>MTTRTTDNPWLDARVLNMAHAGGENEAPANTLYAFKRAVKLGANMLELDVQSTKDDQLVVIHNATVDQTTDGTGKVRDLTFEQVHELDAAYNFIPGRHAVPGEPPESYPLRGVRTGEKKPPPGYQPSDFAIPKLADVLEAFPRTPINIEIKGTSDADIPSFLHNAKLLARLLKKTGRTDFIVTSLNDLAVAKFHLLAPDIPIAPGMAGLAAYFLLGVKPMHGTVALQIPVRYQGLEIATPEFIRRAHADGYAVHVWFSGTAPDDEATYNRIIDSCADGLMPAYPALLERILDERGIERPGRPGVDPCG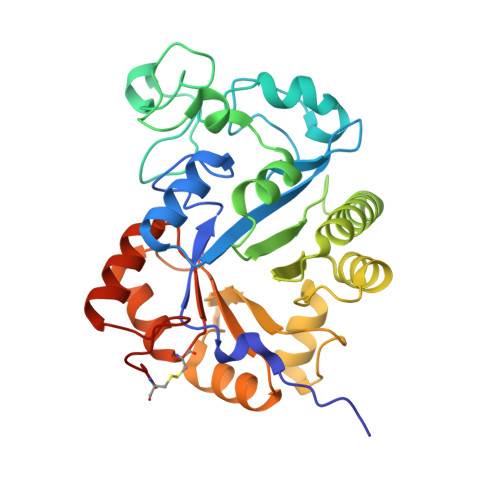HHHHHH[8x]5'-O-[(2-nitrobenzene-1-carbonyl)sulfamoyl]adenosine 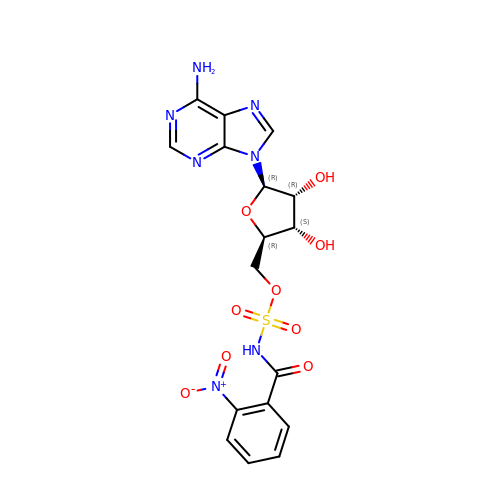| C17 H17 N7 O9 S | OCXRXKRXIAIGOE-CNEMSGBDSA-N> MEINEKLLRQIIEDVLSEMKGSDKPVSFNAPAASAAPQATPPAGDGFLTEVGEARQGTQQDEVIIAVGPAFGLAQTVNIVGIPHKSILREVIAGIEEEGIKARVIRCFKSSDVAFVAVEGNRLSGSGISIGIQSKGTTVIHQQGLPPLSNLELFPQAPLLTL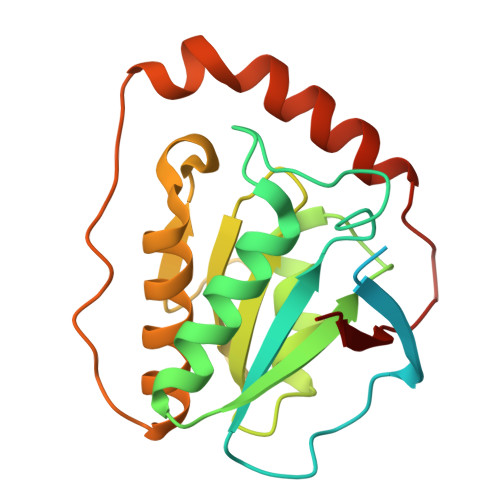ETYRQIGKNAARYAKRESPQPVPTLNDQMARPKYQAKSAILHIKETKYVVTGKNPQELRVAL> QDSTSDLIPAPPLSKVPLQQNFQDNQFHGKWYVVGLAGNRILRDDQHPMNMYATIYELKEDKSYNVTSVISSHKKCEYTIATFVPGSQPGEFTLGNIKSYGDKTSYLVRVVSTDYNQYAVVFFKLAEDNAEFFAITIYGRTKELASELKENFIRFSKSLGLPENHIVFPVPIDQCIDG;> MHVAQPAVVLASSRGIASFV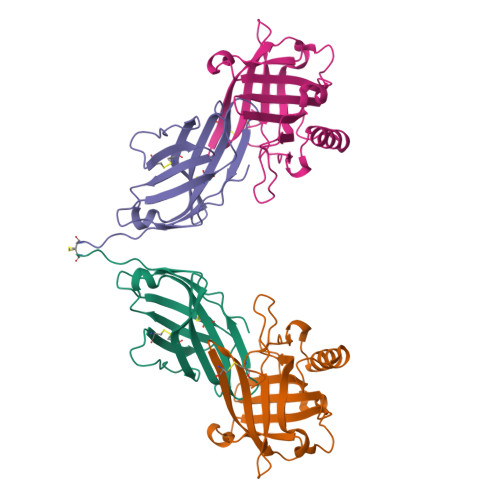CEYASPGKATEVRVTVLRQADSQVTEVCAATYMMGNELTFLDDSICTGTSSGNQVNLTIQGLRAMDTGLYICKVELMYPPPYYLGIGNGTQIYVIDPEPCPDSD>MALKDDAVLIAARGYVYTAAVGTAAPTPSQLKLIDLEHPEAWDRTGWDLVGHTSEDDLPEFGFDGGDSEVRGSWQKKKLREVETEEIADYVVINLTQFDETALELYFGPNQSATPGIFGVKSGSVVNERALLIVIVDNDVRLGFHARKASLKREDAISLATDEFGALPVRATFLDYQSYNLYEWIEEDWFNAVDAPVVYLLDLGGATGGDYTLLVGGKSTGDIAYNANASAIKTAIGAVDDGVAESAWTVTADGSDFEISGPLAVALGV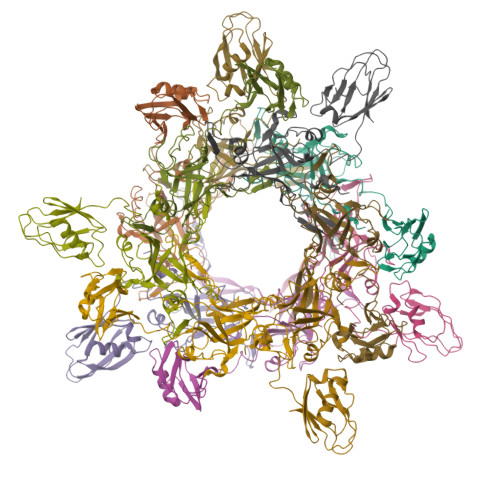DSTTGGSGVTVDVV[12x]>[3x]GCTGGATATATCCAGC

The rational design of small molecules that target specific DNA sequences is a promising strategy to modulate gene expression. This report focuses on a diamidinobenzimidazole compound, whose selective binding to the minor groove of AT DNA sequences holds broad significance in the molecular recognition of AT-rich human promoter sequences. The specialized method of X-ray crystallography was utilized to investigate how the sequence-dependent recognition properties in general, A-tract, and alternating AT sequences affect the binding of diamidinobenzimidazole in the DNA minor groove. A strong and direct hydrogen bond between the N-H of the benzimidazole and an H-bond acceptor atom in the minor groove is essential for DNA recognition in all sequences described. In addition, the diamidine compound specifically utilizes an interfacial water molecule for its DNA binding.

An extended alternate AT sequence (ATATAT) is also described. Here, we report a 16-mer ATATAT-DB1476 complex structure at a resolution of 1.50 Å, with Rwork and Rfree at 25.9 and 29.2%, respectively. The crystal structure has the space group P3121, which is different from all other structures in this study. The DB1476 compound binds in a singular orientation, like AAATTT and ATAT, in the presence of a unique external water molecule that stabilizes the complex at the B-N1. A bifurcated hydrogen bond is observed between the BI-NH and the O2 of T9 and T25, respectively. The C-N4 amidine has a longer than expected bonding distance from their nearest DNA hydrogen bond acceptor. The interfacial water molecule observed at A-N6 does not have an optimum H-bond distance from the DNA. The unusual bonding distances suggest a very dynamic interaction at the amidine ends, and therefore, DB1476 will not bind as strongly to the −ATATAT– (KD = 16 nM) sequences in comparison to −ATAT– (KD = 12 nM). The ATATAT-DB1476 structure utilizes its extensive large water network to stabilize its complex. ATATAT-DB1476 also shows the same twist pattern with a high twist at the TpA step (42°) that is flanked by a lower twist from the two ApT steps (30°), respectively.ethyl 5'-formyl[2,2'-bipyridine]-5-carboxylate 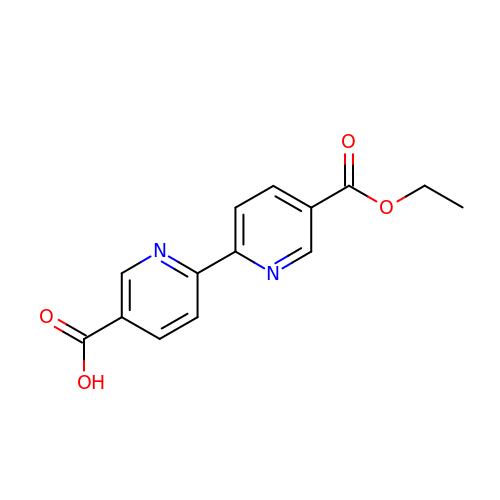| C14 H12 N2 O4 | FZDQJVHCAWGPRW-UHFFFAOYSA-N> MGSDKIHHHHHHNTPREVTLHFLRTAGHPLTRWALQRQPPSPKQLEEEFLKIPSNFVSPEDLDIPGHASKDRYKDILPNPQSRVCLGRAQSQEDGDYIN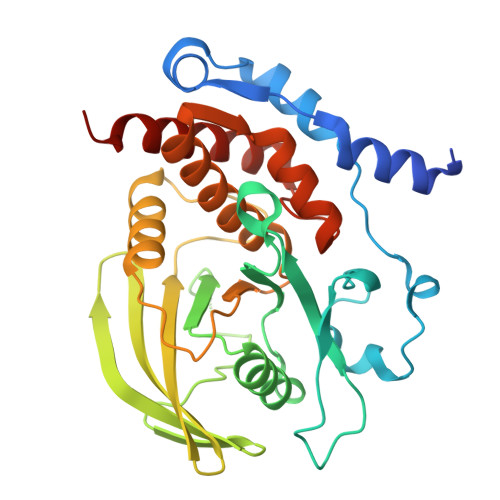ANYIRGYDGKEKVYIATQGPMPNTVSDFWEMVWQEEVSLIVMLTQLREGKEKCVHYWPTEEETYGPFQIRIQDMKECPEYTVRQLTIQYQEERRSVKHILFSAWPDHQTPESAGPLLRLVAEVEESPETAAHPGPIVVHSSAGIGRTGCFIATRIGCQQLKARGEVDILGIVCQLRLDRGGMIQTAEQYQFLHHTLALYAGQLPEEPSP In Escherichia coli, isocitrate dehydrogenase kinase/phosphatase (AceK) is a unique bifunctional enzyme with both protein kinase and phosphatase activities. AceK phosphorylates and dephosphorylates isocitrate dehydrogenase (IDH) in response to nutrient availability. The reversible phosphorylation results in the inactivation or activation of IDH, which regulates the branch point between the Krebs cycle and the glyoxylate bypass. The C-terminal part (kinase domain, KD) forms a typical kinase scaffold responsible for the functions of kinase, phosphatase and ATPase, which binds to adenosine triphosphate (ATP) or adenosine diphosphate (ADP).

In this work, we report the crystal structure of AceK in complex with Mn2+ and ADP. Two Mn2+ ions were found in the active site of AceK, which is different from the previous structures. For the two metal ions (designated M1 and M2) found in the catalytic center of AceK-Mn2+ the catalytic core displays an identical position of M1 compared to AceK-Mg2+. Two ions (M1, M2) separated by 3.9 Å are coordinated by the conserved aspartic acid residues Asp475, Asp477, and Asn462, ADP and water molecules. Each ion is hexa-coordinated by oxygen atoms from protein residues, ADP, and water molecules. The environments of the two metal ions in the AceK catalytic site differ; Mn2+ at M1 forms direct coordination with the carboxylate groups of two residues: Asp475, Asn462, which is the same with Mg2+ in the AceK-Mg2+ structure; while Mn2+ at M2 forms direct contact with carboxylate side chains of Asp477 and Asp475. In the Mn2+-binding site of AceK, the two metal ions are both bridged by Asp475, whereas Asp477 is only coordinated to the M2 metal ion. In the structure of AceK-Mn2+, the M2 metal ion indirectly interacts with Glu478 through water-mediated hydrogen bonds. The calculated numbers of binding sites were 2.37 for Mn2+ and 1.36 for Mg2+, which indicated that there is only one Mg2+ (presumably M1) binding to AceK WT, whereas two Mn2+ (presumably M1 and M2) binding to AceK WT. Results of the enzymatic activity of AceK with Mg2+ and Mn2+ revealed that the phosphatase activity of AceK-Mn2+ was higher than that of AceK-Mg2+, whereas the kinase activity was almost unchanged.

>[2x]MPRGLELLIAQTILQGFDAQYGRFLEVTSGAQQRFEQADWHAVQQAMKNRIHLYDHHVGLVVEQLRCITNGQSTDAEFLLRVKEHYTRLLPDYPRFEIAESFFNSVYCRLFDHRSLTPERLFIFSSQPERRFRTIPRPLAKDFHPDHGWESLLMRVISDLPLRLHWQNKSRDIHYIIRHLTETLGPENLSKSHLQVANELFYRNKAAWLVGKLITPSGTLPFLLPIHQTDDGELFIDTCLTTTAEASIVFGFARSYFMVYAPLPAALVEWLREILPGKTTAELYMAIGCQKHAKTESYREYLVYLQGCNEQFIEAPGIRGMVMLVFTLPGFDRVFKVIKDKFAPQKEMSAAHVRACYQLVKEHDRVGRMADTQEFENFVLEKRHISPALMELLLQEAAEKITDLGEQIVIRHLYIERRMVPLNIWLEQVEGQQLRDAIEEYGNAIRQLAAANIFPGDMLFKNFGVTRHGRVVFYDYDEICYMTEVNFRDIPPPRYPEDELASEPWYSVSPGDVFPEEFRHWLCADPRIGPLFEEMHADLFRADYWRALQNRIREGHVEDVYAYRRRQRFSVRYGEMLF> MWSKVFTPLLTHRLTPAEKFPQLQLRVGQQRRVTCGRQLSIPLSSFDSHSLDFARREIEPGSVVELRDADHRKLLALAFYEPALLRVDIFHHTPKVVTDLPRISEDFFVNRVKEAWGRRQSVFRHVRTGSTNAYRVVNGYADGVPSLYVDLFSSSFARVVATSAGAERIVPAVTELLRQHGVEEVLLDTPHLKDHEKLTLITPTITLPETYMENGASNMWLPRDEYPTTSSNRWLINTAHRRIRAVLRDLCHGKRVLCVNDRGGAAALQAVMTAKSVVFAESDESLLNRVRENLVANHASAVFNTCETTNSPIEELSMRQQDVVFLEHRFDTLSSPEQWQNLLKVMLFRGVCGKGSIVVVAQEVALLGMHDYVASGGGVAASVVRATRSEMFNVFNRVTAEH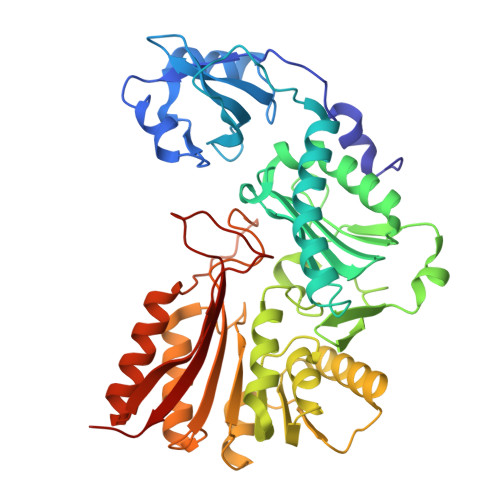GLRARLLRFFGPSIDYPTLPAVEAGCYSYAFLLELAS> SNAMTEKIYDAIVVGAGFSGLVAARELSAQGRSVLIIEARHRLGGRTHVVNFLGRPVEIGGAGVHWCQPHVFAEMQRYGFGFKEAPLADLDKAYMVFADGQKIDVPPATFDEEYTTAFEKFCSRSRELFPRPYSPLDNHEVSNLDGVSARDHLESLGLNELQLASMNAELTLYGGAPTTELSYPSFVKFHALASWDTITFTDSEKRYHVQGGTNALCQAIFDDCRADSEFGVPVEAVAQTDNGVTVTLADKRVF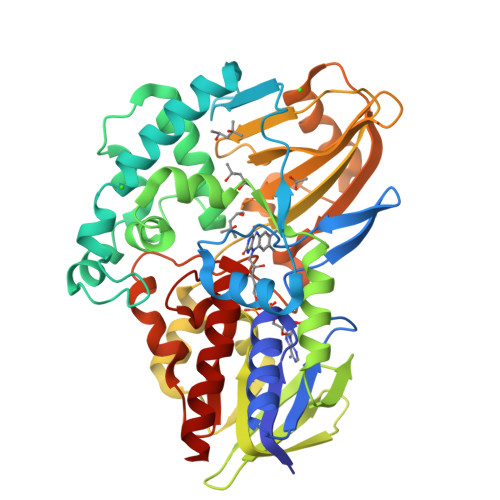RALTCVLTLPTKVYADVRFEPPLPPEKRAFIEHAEMADGAELYVHVRQNLGNTFTFCDDPNPFNAVQTYAYDDELGTILKITIGRQSLINLENFDAIAAEIRKIHGDVEVLEALPYNWAMDEYARTSYPAMRKGWFSRYKDMAKPENRLFFAGSATADGWHEYIDGAIESGIRVGREIRHFMKATA> MAASDEVNLIESRTVVPLNTWVLISNFKVAYNILRRPDGTFNRHLAEYLDRKVTANANPVDGVFSFDVLIDRRINLLSRVYRPAYADQEQPPSILDLEKPVDGDIVPVILFFHGGSFAHSSANSAIYDTLCRRLVGLCKCVVVSVNYRRAPENPYPCAYDDGWIALNWVNSRSWLKSKKDSKVHIFLAGDSSGGNIAH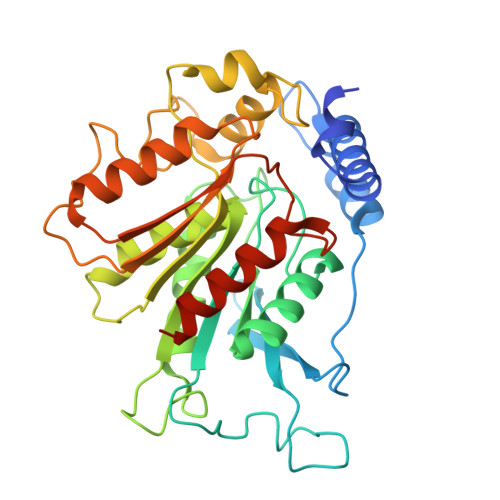NVALRAGESGIDVLGNILLNPMFGGNERTESEKSLDGKYFVTVRDRDWYWKAFLPEGEDREHPACNPFSPRGKSLEGVSFPKSLVVVAGLDLIRDWQLAYAEGLKKAGQEVKLMHLEKATVGFYLLPNNNHFHNVMDEISAFVNAECGGDYKDDDDK> MDFLTSTLLSGILYDGFKNGVAITTGFLKEKL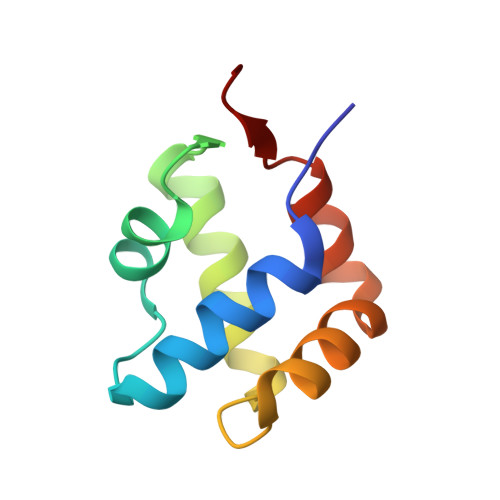HGWIVDDTLLETLAYKVNTLELKDYGEHVIERKLNESSEIQQILKLIQPEQN>GAMLYLEDYLEMIEQLPMDLRDRFTEMREMDLQVQNAMDQLEQRVSEFFMNAKKNKPEWREEQMASIKKDYYKALEDADEKVQLANQIYDLVDRHLRKLDQEL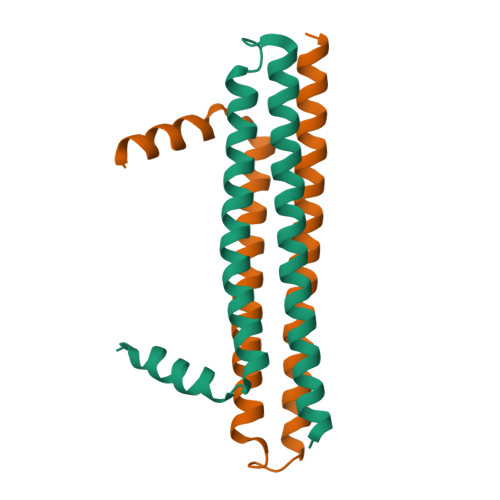A[2x]> HMELFAELRRQGVAPTVVTYNTLIDGLCKAGKLDEALKLFEEMVEKGIKPDEFTFSSVLKACARLGALELGKQIHGYVIKSGFEGNVVVYNALIDMYSKCGLLEEARKVFDEMPEKDVVTYNTLIDGLCKAGKLDEALKLFEEMVEKGIKPDEFTFSSVLKACARLGALELGKQIHGYVIKSGFESNVVVYNALIDMYSKCGLLEEARKVFDEMPEKDVVTYNTLIDGLCKAGKLDEALKLFEEMVEKGIKPDEFTFSSVLKACARLGALELGKQIHGYVIKSGFESNVVVYNALIDMYSKCGLLEEARKVFDEMPEKDELTYRRVVESYCRAKRFELEHHHHH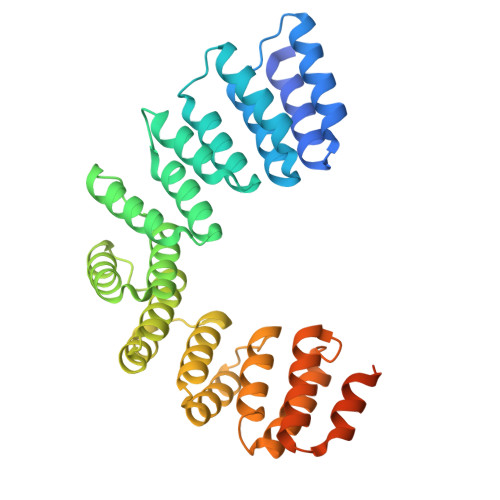HHH>[5x]GQDMVSPPPPIADEPLTVNTGIYLIECYSLDDKAETFKVNAFLSLSWKDRRLAFDPVRSGVRVKTYEPEAIWIPEIRFVNVENARDAD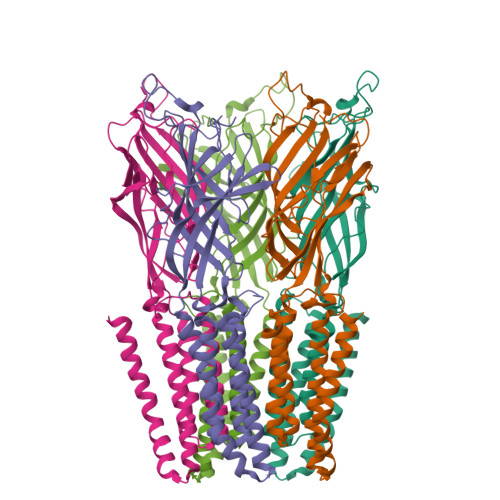VVDISVSPDGTVQYLERFSARVLSPLDFRRYPFDSQTLHIYLIVRSVDTRNIVLAVDLEKVGKNDDVFLTGWDIESFTAVVKPANFALEDRLESKLDYQLRISRQYFSYIPNIILPMLFILFISWTAFWSTSYDANVTLVVSTLIAHIAFNILVETNLPKTPYMTYTGAIIFMIYLFYFVAVIEVTVQHYLKVESQPARAASITRASRIAFPVVFLLANIILAFLFFGF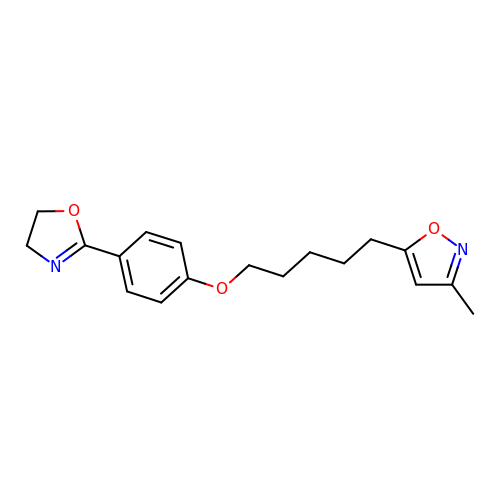5-(5-(4-(4,5-DIHYDRO-2-OXAZOLY)PHENOXY)PENTYL)-3-METHYL ISOXAZOLE | C18 H22 N2 O3 | IWZDYGHUSXWPPM-UHFFFAOYSA-N ethyl (3~{S},7~{R},10~{R},11~{R},13~{S})-4-[(3~{S},6~{R},8~{a}~{S})-1'-[(2~{S})-2-acetamido-3-(2-chlorophenyl)propanoyl]-5-oxidanylidene-spiro[1,2,3,8~{a}-tetrahydroindolizine-6,2'-pyrrolidine]-3-yl]carbonyl-11-ethyl-2-oxidanylidene-1,4-diazatricyclo[8.3.0.0^{3,7}]tridec-8-ene-13-carboxylate 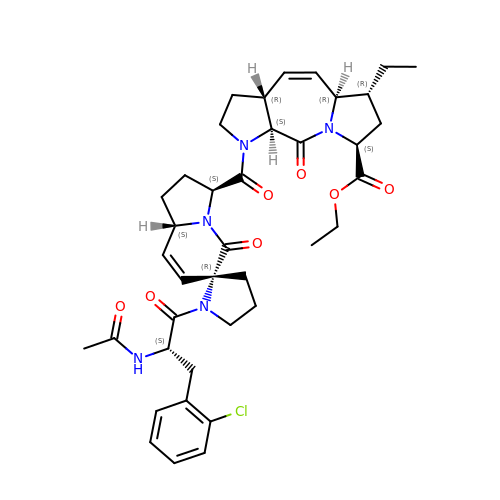| C39 H48 Cl N5 O7 | UDCSMDQSVHUJOU-FHKBVFMSSA-N> VNGAGLLQTVWGPVCELTSELDGQAGAALKKEQEMLAKINDMQMAQLRAAIYL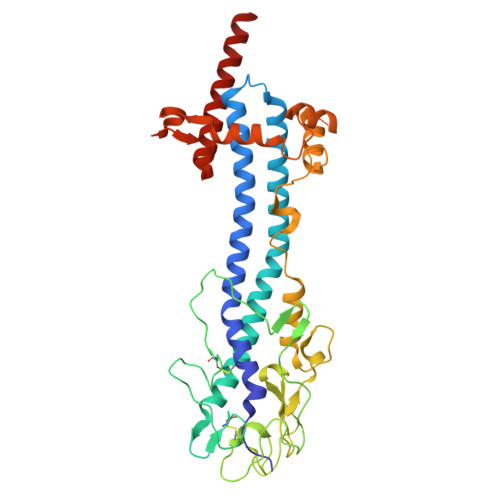AKNPSTPHQNALAVLTAYYAERAGSGKAYFLHALPKAVDSIRRAAYLKGHLDEYLNLLEKSSGGNNKCLVTTDDATVATRGGDQKLAGKNCKLSLSPLKPVDAALTYITKAGVGKLRYDDGGAGGNAVTPSKSGVHACKLLIAHNTAGYGDGGGVTADIDVFAGYMKVKATDAEPKLAAKSDLEEGGGGGAEAWKALHTAIKQEADAEAAELTNETGKLGERRHFLAAATNVLGTGAAGTGNAGRAAVEAAFGSDSEGGDRKIIELIEKELIVKGTANRDADESLGNIKTLKELGELLSYFQLKNSNTINELRNKLK>[2x]GNSDDARTSIEQRSNAVSQVLLGIFSYVRWPKEPAVLQLCVVGPTEYADGLLRGMVQANGRRVHAERRAVDNPDLGTLCNVIYLGVVDERERQQVFRSLAGHPVLSISERGTECSVGSMFCLNVGGPRITFEANLDSIARSGVRVHPS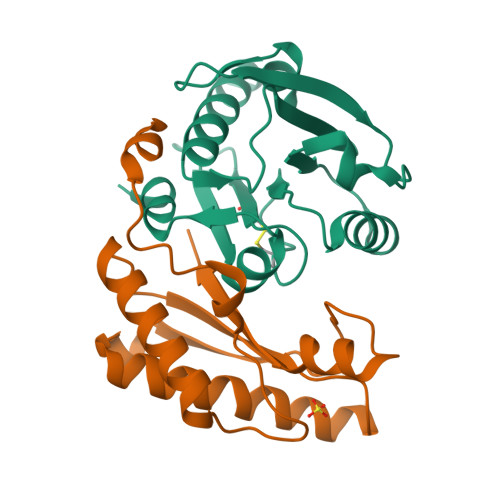VLKLARRQATP;>[2x]GLSAEQIAVPQEQGFELRDEGWEFGMSSKVLFGNNLDRLNPDSRNTLTKIARALLAVDIDKVRLEGHTDNYGDEGYNQKLSERRAESVAAVFREAGMPAANIEVRGLGMSKPVADNKTRAGRSENRRVAIIVPAE> MHHHHHHVIGLSTGSDDDDVEVIGGVDPRLIAVQENDSDESSLTDLVEQPAKVMRIGTM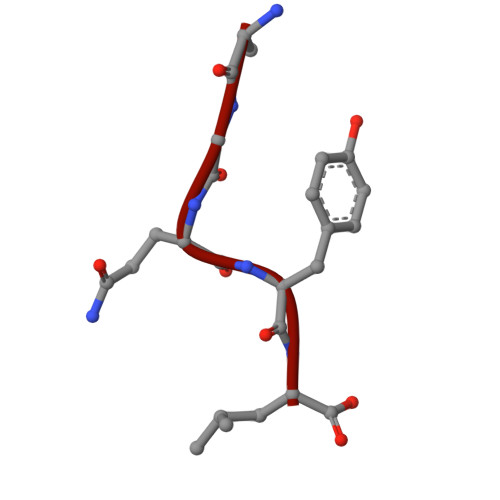IKQLLEEVRAAPLDEASRNRLRDIHATSIRELEDGLAPELREELDRLTLPFNEDAVPSDAELRIAQAQLVGWLEGLFHGIQTALFAQQMAARAQLQQMRQGALPPGVGKSGQHGHGTGQYL3-[(1E)-3-carboxyprop-1-en-1-yl]benzene-1,2-dicarboxylic acid | C12 H10 O6 | 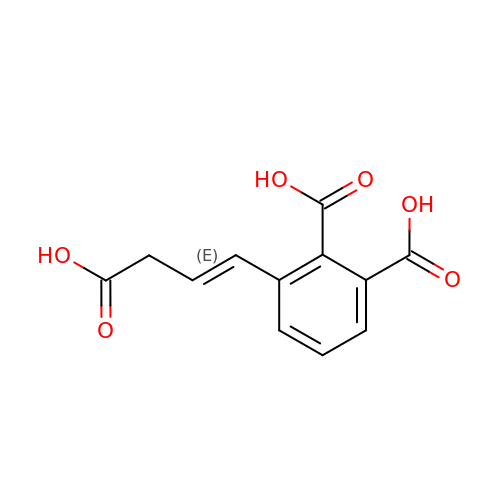IVICCMHKRTYMTD-DUXPYHPUSA-N>[2x]MFTGSIVAIVTPMDEKGNVCRASLK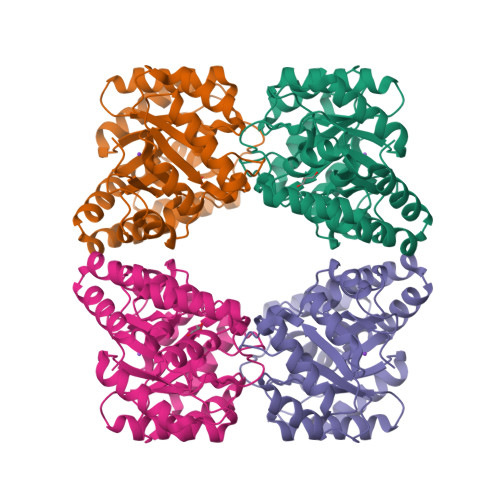KLIDYHVASGTSAIVSVGTTGEWATLNHDEHADVVMMTLDLADGRIPVIAGTGANATAEAISLTQRFNDSGIVGCLTVTPYYNRPSQEGLYQHFKAIAEHTDLPQILYNVPSRTGCDLLPETVGRLAKVKNIIGIKEATGNLTRVNQIKELVSDDFVLLSGDDASALDFMQLGGHGVISVTANVAARDMAQMCKLAAEGHFAEARVINQRLMPLHNKLFVEPNPIPVKWACKELGLVATDTLRLPMTPITDSGRETVRAALKHAGLL> SGASSAVGGSTRSPSPVDPKRGAVQPRYFITTSLTEKERNSVMEAIQKLGQRAVLVDNKVDEILPLNTTHIVLRGPPRSVAALCGVVSSKWLVQPSYVFDSLGAGFWLDEEVEGGLRYFPPPLRCQRFLLTMPEGVVKTMLQRVVEFGGGEVVGTKRNGSSNDQDVVVVSSGDELLRFAISRD

KKT4 is a multi-domain kinetochore protein specific to kinetoplastids, such as Trypanosoma brucei. It lacks significant sequence similarity to known kinetochore proteins in other eukaryotes. KKT4 is an essential kinetochore component and has microtubule-binding activity. We recently reported the X-ray structure of the KKT4 C-terminal region (see Fig. 1A for the domain organization of KKT4), showing that it has a tandem BRCT (BRCA1 C Terminus) domain fold.

Our recent X-ray structure of the C-terminal region of KKT4 shows that it has a tandem BRCT (BRCA1 C Terminus) domain fold with a sulfate ion bound in a typical binding site for a phosphorylated serine or threonine. Our initial analysis suggested that the BRCT domain in KKT4 is involved in phosphopeptide binding. We show that the BRCT domain can bind phosphate ions in solution using residues involved in sulfate ion binding in the X-ray structure. We have confirmed that in solution the BRCT domain binds phosphate ion in the sulfate ion binding site previously identified by X-ray crystallography. Mutating the residues involved in phosphate ion binding in T. brucei KKT4 BRCT results in growth defects confirming the importance of the BRCT phosphopeptide-binding activity in vivo. The in vivo importance of phosphopeptide binding also demonstrates the potential for rational drug design to target neglected tropical diseases caused by kinetoplastid parasites.>[2x]MYQAGGTIRSLLDKVAEQEYLLPAIQREFVWRPEQICRLFDSLLQGYPFGTFLFWKIKPENRDSYQFYQFMQHYHERDNYHCENVTQLPEREFIAVLDGQQRITALNIGLRGSFAWKLTGKWWSNDDAFPVRRLHLNLLSKPDLETGSMYDFEFLTDDKASLDASEQYWFRVGRIMEEEEDALIDEVADDARLSSEQRKEARSTLRHLYRTIHDKDKISFYEESDQSLERVLNIFIRMNSGGTTLSYSDLLLSIAVAQWSSLDAREEIHALVDEMNRVGDGFNVSKDLVLKAGLMLSDIGSVGFKVENFNKENMAILEKNWTPIRDALLLSMQLLASFGFNAQNLRATSAILPLAYYLHHRKLTASYLSRVEYAVDRECIRNWLIRSLLKASGIWGSGLDTLLTMLRSDIKQSGDTGFPLAKIEATMQQRGKSLRFDPEEISELAQLDYGNPRTFALLTLLFPGFDFSRHFHVDHIYPKGLFTRNKLAKVGVPAEQLDELIEASNKLPNLQLLEGTINNQKRQKMPHEWYAQQWPDVNARQAHLQSQAITSLPEQLNQFMDFYRERQETLLARIRTALQPASSVETE

Using a suite of thirty environmentally-isolated coliphages, we demonstrate multi-layered and robust phage protection provided by a plasmid-encoded defence island that expresses both a type I BREX system and the novel GmrSD-family type IV DNA modification-dependent restriction enzyme, BrxU. The BrxU protein contains DUF262 and DUF1524 domains, and shares 13% amino acid sequence identity with the single polypeptide type IV restriction enzyme GmrSD. Here, we have shown that BrxU is a promiscuous enzyme that uses a range of nucleotide and metal co-factors to recognise and cleave DNA that contains any of at least three different modifications, and this activity is dependent on the initial nucleotide-driven dissociation of BrxU dimers, and subsequent nucleotide hydrolysis. Our BrxU structures are the first for the GmrSD family, providing the highest resolution detail for the widespread DUF262 and DUF1524 domains.

In order to better understand the biochemical data, the dimeric structure of BrxU was solved to 2.12 Å. The N-terminal DUF262 domain of BrxU is connected to the C-terminal DUF1524 domain by a flexible linker. These linkers entwine in the observed dimer, and then a loop from each N-terminal domain connects with the corresponding protomeric C-terminal domain (bridged by a glycerol molecule in the structure), such that the dimer is, in effect, two interlocked circles. The relative rotation between N- and C-terminal domains is easily observed from a top-down view, and generates a cleft that runs diagonally across the dimer. This cleft is ∼21 Å wide, and surface electrostatics show clear patches of electropositivity throughout, with the N-terminal domains as the floor and the C-terminal domains forming the walls. Within our structure, the position of the γ-phosphate has been taken by a sulphate ion that is bound by R102, and nucleotide binding has been prevented by proximity of an α-helix and linker from the opposing protomer that fill the corresponding space where a nucleotide might bind, also blocking S42 of the RLFDS motif. Within the C-terminal DUF1524 domain, D474 and H475 of the BrxU DHIYP nuclease motif are positioned on the surface of the DUF1524 domain to form part of the cleft wall within BrxU. A glycerol molecule bridges the DUF1524 with a loop extending from the DUF262 domain, and an additional sulphate ion and chloride ion were observed bound by looped regions of DUF1524. Despite setting crystals in the presence of AMP-PnP, no nucleotide ligand was detected in the structure. It therefore makes sense that our crystals contain BrxU dimers, without bound nucleotide.>[2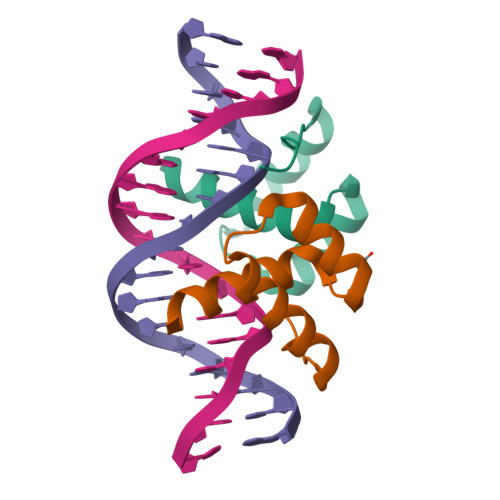x]GPAREGARRKRTTFNKTQLEILVKSFNKDPYPGIGVREHLASLIQIPESRIQVWFQNRRARQLGQKKKLEV> P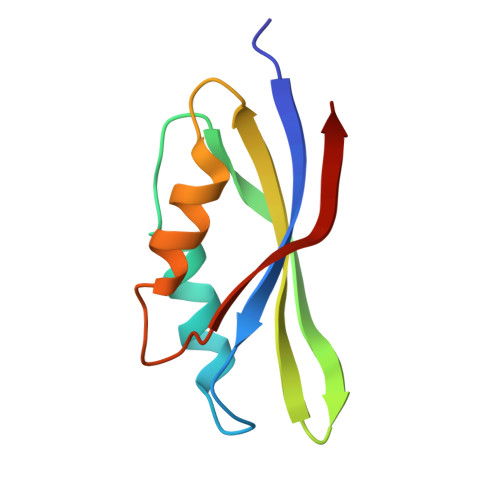AAKSIVTLDVKPWDDETNLEEMVANVKAIEMEGLTWGAHQFIPIGFGIKKLQINCVVEDDKVSLDDLQQSIEEDEDHVQSTDIAAMQKL>[3x]GSHMFTGLNTPS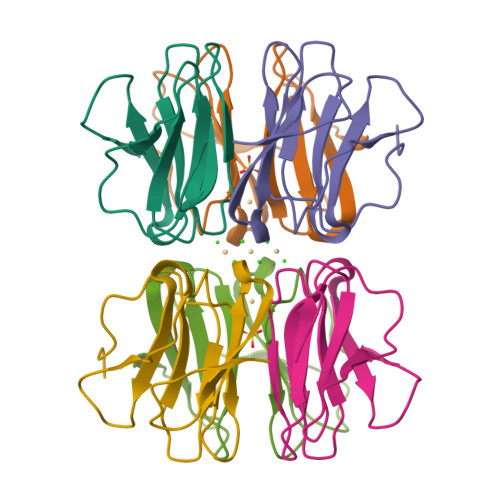GVAVDSAGTVYVTDHGNNRVVKLAAGSNTQTVLPFTGLNTPHGVAVDSAGTVYVTDHGNNRVVKLAAGSNTQTVL(2E)-3,7-dimethylocta-2,6-dienoic 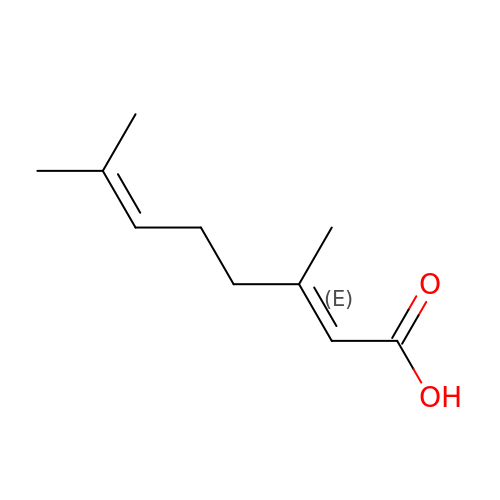acid | C10 H16 O2 | ZHYZQXUYZJNEHD-VQHVLOKHSA-N>MTPPIISPESFEALRRMRAAEPTMVAERFKQRRKRELLGEDGKLFIVAADHPARGALAVGDNETAMANRYELLERMAIALSRPGVDGVLGTPDIIDDLAALGLLDDKIVVGSMNRGGLRGASFEMDDRYTGYNVSSMVDRGVDFAKTLVRINLSDAGTAPTLEATAHAVNEAAAAQLPIMLEPFMSNWVNGKVVNDLSTDAVIQSVAIAAGLGNDSSYTWMKLPVVEEMERVMESTTMPTLLLGGEGGNDPDATFASWEHALTLPGVRGLTVGRTLLYPQDGDVAAAVDTAARLVHTDIQQ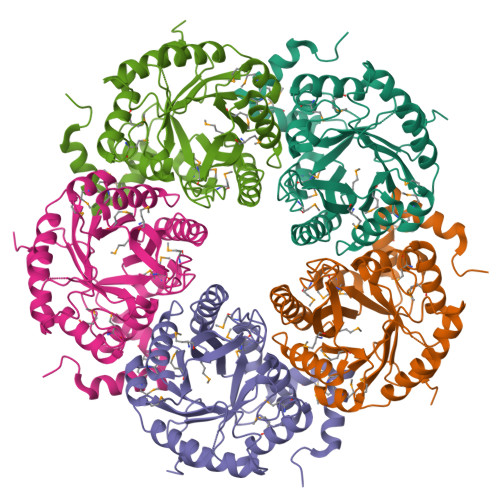FTSQSI[10x]To elucidate the molecular features encoded by these conserved elements, we solved the crystal structures of Arabidopsis thaliana SOBER1 and Zea mays B6T1C9, each representing a different clade in the phylogenetic tree. Both proteins fold into a canonical α/β hydrolase architecture and superpose with a root-mean-square deviation (RMSD) of atomic positions of 1.54 Å over 210 amino acid residues. We found that a loop constituting the hydrophobic tunnel lid is the major component determining substrate turnover rate and substrate specificity.

To investigate if loop flexibility is directly dependent on the strength of the hydrophobic anchor, we designed a mutant, in which we substituted the phenylalanine, which is the most hydrophobic amino acid on the Hoop-Woods scale, with a leucine (AtSOBER1 F65L). While the mutant crystallized in the same space group and cell dimensions, we found the loop B-factors significantly increased when compared to wild type AtSOBER1, indicating that its flexibility had improved just by changing the residue that anchors the loop inside the hydrophobic tunnel. While the catalytic efficiency was decreased in AtSOBER1 by substituting the phenylalanine anchor F65 by a leucine residue, the opposite effect was observed upon replacement of L110 by a phenylalanine residue in AtTIPSY1. We hypothesize that a more flexible lid-loop renders the surface created by L63 in AtSOBER1 less rigid and therefore less suitable for deacetylation. For pNP butyrate (C4), valerate (C5), and hexanoate (C6), we measured increased catalytic efficiencies after introducing a weaker anchor (AtSOBER1 F65L) and a decrease in AtTIPSY1 L110F. The observed differences in catalytic efficiencies for those C4–C6 chains are mostly resulting from higher or lower turnover numbers rather than significantly different substrate affinities. This suggests that the strength of the hydrophobic anchor determines the flexibility of the lid-loop and that a more flexible loop leads to a significant increase in product release. Our attempts to turn a SOBER1 protein into a TIPSY1 protein by altering the hydrophobic anchor (AtSOBER1 F65L) were a partial success. Weakening the anchor allowed the protein to hydrolyze para-nitrophenyl hexanoate, like AtTIPSY1 is able to. AtSOBER1 F65L also displayed higher affinities to longer-chain substrates and the lowest affinity to para-nitrophenyl acetate, a pattern opposite to wild type.

> GPMARTFILWLHGLGDSGPANEPIQTQFKSSELSNASWLFPSAPFNPVTCNNGAVMRSWFDVPELPLKVGSPIDESSVLEAVKNVHAIIDQEIAEGTNPENVFICGLSQGGALTLASVLLYPKTLGGGAVLSGWVPFTSSIISQFPEEAKKTPILWSHGTDDRMVLFEAGQAALPFLKEAGVTCEFKAYPGLGHSISNKELKYIESWIKRRLKGSSSTCLQLNCLKEMFH>APSRKFFVGGNWKMNGRKQSLGELIGTLNAAKVPADTEVVCAPPTAYIDFARQKLDPKIAVAAQNCYKVTNGAFTGEISPGMIKDCGATWVVLGHSERRHVFGESDELIGQKVAHALAEGLGVIACIGEKLDEREAGITEKVVFEQTKVIADNV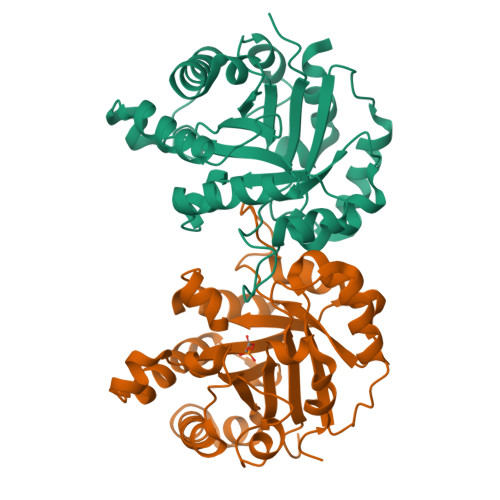KDWSKVVLAYEPVWAIGTGKTATPQQAQEVHEKLRGWLKSNVSDAVAQSTRIIYGGSVTGATCKELASQPDVDGFLVGGASLKPEFVDIINAKQ[2x]>MRSRRVDVMDVMNRLILAMDLMNRDDALRVTGEVREYIDTVKIGYPLVLSEGMDIIAEFRKRFGCRIIADFKVADIPETNEKICRATFKAGADAIIVHGFPGADSVRACLNVAEEMGREVFLLTEMSHPGAEMFIQGAADEIARMGVDLGVKNYVGPSTRPERLS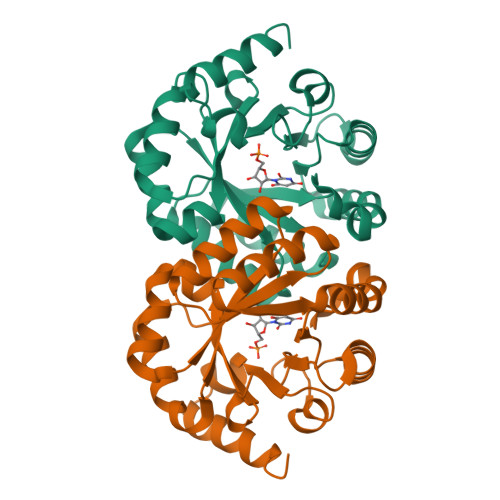RLREIIGQDSFLISPGVGAQGGDPGETLRFADAIIVGRSIYLADNPAAAAAGFIESIKDLLNP[2x]> MEDEIRKAAEILAKSKHAVVFTGAGISAESGIPTF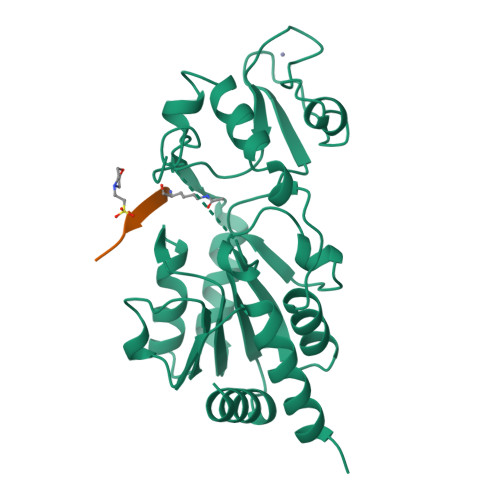RGEDGLWRKYDPEEVASISGFKRNPRAFWEFSMEMKDKLFAEPNPAHYAIAELERMGIVKAVITQNIDMLHQRAGSRRVLELHGSMDKLDCLDCHETYDWSEFVEDFNKGEIPRCRKCGSYYVKPRVVLFGEPLPQRTLFEAIEEAKHCDAFMVVGSSLVVYPAAELPYIAKKAGAKMIIVNAEPTMADPIFDVKIIGKAGEVLPKIVEEVKRLRSEK;> KKGQSTSRHKKLMFKTEG> MKHHHHHHHMVSTLKPLKIGKHTIKFPIFQGGMGVGISWDELAGNVAKEGALGVISAVGTGYYKNMRFVERIVAKKPFEALNFYSKKALNEIFANARKICGNNPLGANILYAINDYGRVLRDSCEAGANIIITGAGLPTNMPEFAKDFSDVALIP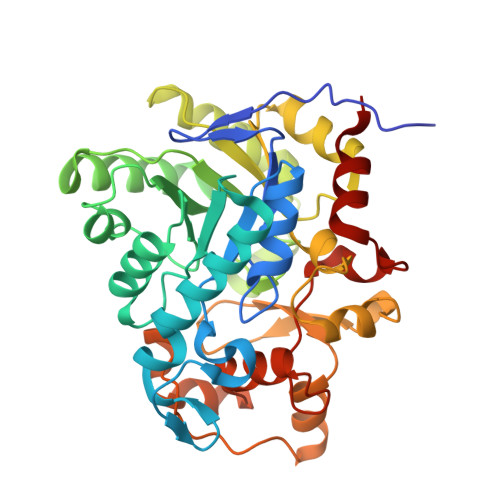IISSAKALKILCKRWSDRYKRIPDAFIVEGPLSGGHQGFKYEDCFKEEFRLENLVPKVVEASKEWGNIPIIAAGGIWDRKDIDTMLSLGASGVQMATRFLGTKECDAKVYADLLPTLKKEDILLIKSPVGYPARAINTGVIKRIEEGNAPKIACVSNCVAPCNRGEEAKKVGYCIADGLGRSYLGNREEGLYFTGANGYRVDKIISVHELIKELTEG> MATVGGIKEVDGNQNSLEI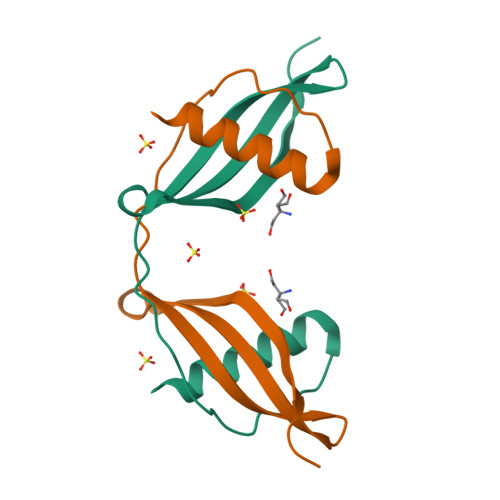ESLARYAVDEHNKKQNSLLQFEKVVNTKQQVVSGTIYIITLEAVDGGKKKVYEAKVWEKPWMNFKELQEFKLIGDAPSGSSA(1~{R},2~{R},3~{S},4~{R},5~{R},6~{R})-5-(hydroxymethyl)-7-azabicyclo[4.1.0]heptane-2,3,4-triol 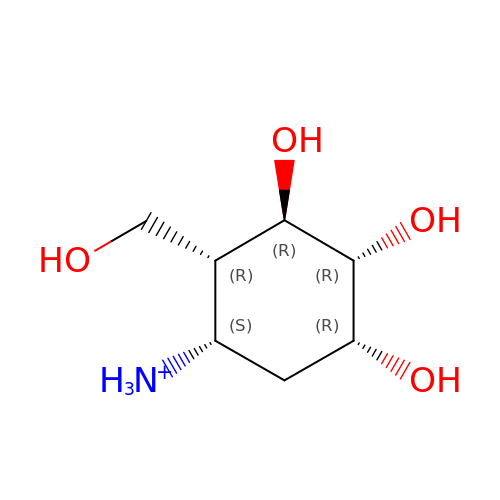| C7 H16 N O4 | FGLYJEXIORSHSO-PAMBMQIZSA-O> DYVLYKDATKPVEDRVADLLGRMTLAEKIGQMTQIERLVATPDVLRDNFIGSLLSGGGSVPRKGATAKEWQDMVDGFQKACMSTRLGIPMIYGIDAVHGQNNVYGATIFPHNVGLGATRDPYLVKRIGEATALEVRATGIQYAFAPCIAVCRDPRWGRCYESYSEDRRIVQSMTELIPGLQGDVPKDFTSGMPFVAGKNKVAACAKHFVGDGGTVDGINENNTIINREGLMNIHMPAYKNAMDKGVSTVMISYSSWNGVKMHANQDLVTGYLKDTLKFKGFVISDWEGIDRITTPAGSDYSYSVKASILAGLDMIMVPNKYQQFISILTGHVNGGVIPMSRIDDAVTRILRVKFTMGLFENPYADPAMAEQLGKQEHRDLAREAARKSLVLLKNGKTSTDAPLLPLPKKAPKILVAGSHADNLGYQCGGWTIEWQGDTGRTTVGTTILEAVKAAVDPSTVVVFAENPDAEFVKSGGFSYAIVAVGEHPYTETKGDNLNLTIPEPGLSTVQAVCGGVRCATVLISGRPVVVQPL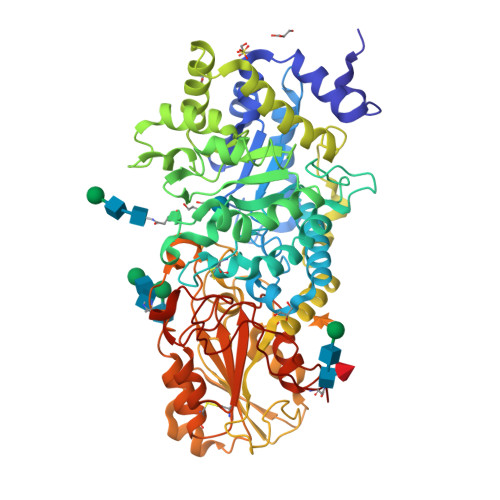LAASDALVAAWLPGSEGQGVTDALFGDFGFTGRLPRTWFKSVDQLPMNVGDAHYDPLFRLGYGLTTNATKKY> YNGQSE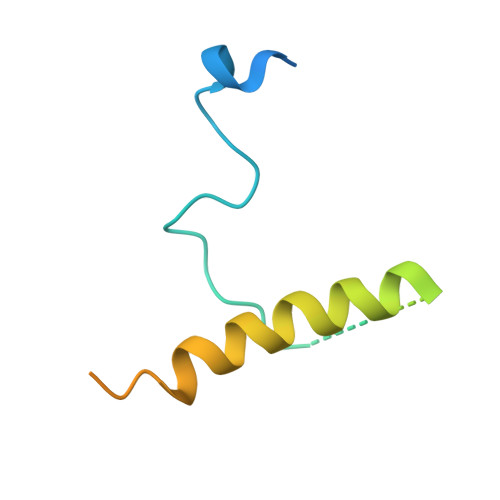TSQQPETPVFNTLPMMGKASPVSLGVPSEATANNGQQQQVQEQRRRINAMLQDYELQRRLHSEQLQFEQAQTQQAAVQVPGIQTLGTQSQ>MHHHHHHHHAMSNSKFNVRLLTEIAFMAALAFIISLIPNTVYGWIIVEIACIPILLLS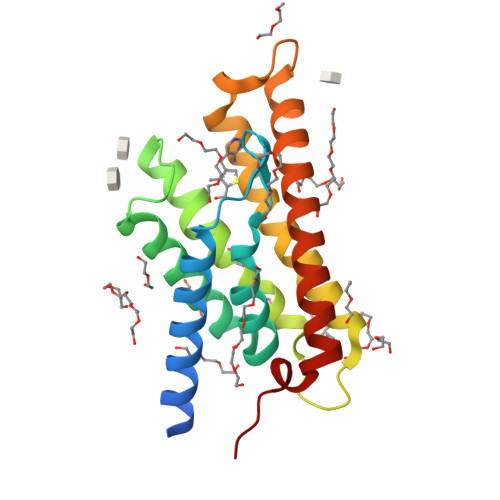LRRGLTAGLVGGLIWGILSMITGHAYILSLSQAFLEYLVAPVSLGIAGLFRQKTAPLKLAPVLLGTFVAVLLKYFFHFIAGIIFWSQYAWKGWGAVAYSLAVNGISGILTAIAAFVILIIFVKKFPKLFIHSNY[2x]> MAKELDATNISIDKVVGAGEFGEVCSGRLKLPSKKEISVAIKTLKVGYTEKQRRDFLGEASIMGQFDHPNIIRLEGVVTKSKPVMIVTEYMENGSLDSFLRKHDAQFTVIQLVGMLRGIASGMKYLSDMGYVHRDLAARNILINSNLVCKVSDFGLSRVLEDDPEAAYTTRGGKIPIRWTSPEAIAYRKFTSASDVWSYGIVLWEVMSYGERPYWEMSNQDVIKAVDEGYRLPPPMDCPAALYQL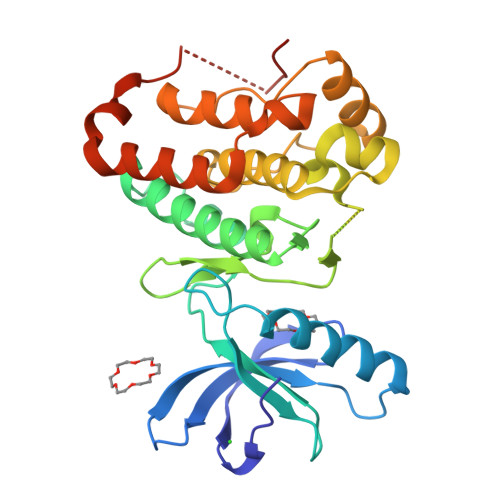MLDCWQKDRNNRPKFEQIVSILDKLIRNPGSLKIITSAAARPSNLLLDLEHHHHHH>[4x]MASMTGGQQMGRGSMA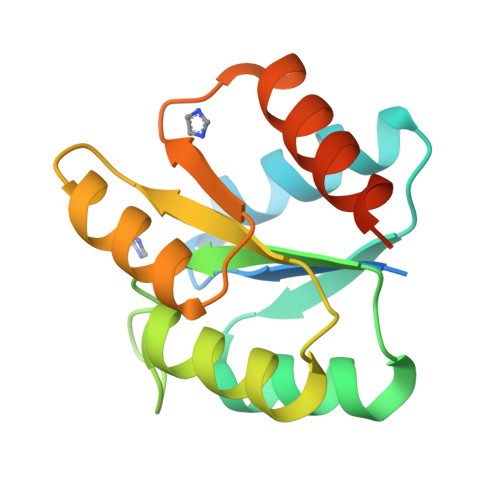ADILVVDDEVDIRDLVAGILSDEGHETRTAFDADSALAAINDRAPRLVFLDIWLQGSRLDGLALLDEIKKQHPELPVVMISGHGNIETAVSAIRRGAYDFIEKPFKADRLILVAERALETSKLKLEHHHHHH> MFARLIRYFQEARAELARVTWPTREQVVEGTQAILLFTLAFMVILGLYDTVFRFLIGLLR;> MVKAFWSALQIPELRQRVLFTLLVLAAYRLGAFIPTPGVDLDKIQEFLRTAQGGVFGIINLFSGGNFERFSIFALGIMPY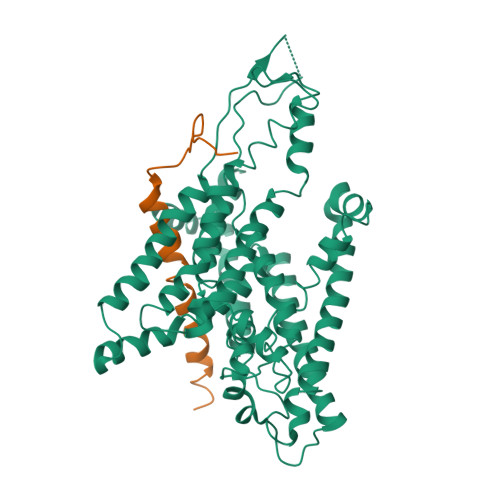ITAAIIMQILVTVVPALEKLSKEGEEGRRIINQYTRIGGIALGAFQGFFLATAFLGAEGGRFLLPGWSPGPFFWFVVVVTQVAGIALLLWMAERITEYGIGNGTSLIIFAGIVVEWLPQILRTIGLIRTGEVNLVAFLFFLAFIVLAFAGMAAVQQAERRIPVQYARKVVGGRVYGGQATYIPIKLNAAGVIPIIFAAAILQIPIFLAAPFQDNPVLQGIANFFNPTRPSGLFIEVLLVILFTYVYTAVQFDPKRIAESLREYGGFIPGIRPGEPTVKFLEHIVSRLTLWGALFLGLVTLLPQIIQNLTGIHSIAFSGIGLLIVVGVALDTLRQVESQLMLRSYEGFLSRGRLR>[2x]MAIVKATDQSFSAETSEGVVLADFWAPWCGPSKMIAPVLEELDQEMGDKLKIVKIDVDENQETAGKYGVMSIPTLLVLKDGEVVETSVGFKPKEALQELVNKHLLEHHHHHH

Thioredoxin is a ubiquitous protein that is present in nearly all known organisms from archaea to humans. In its active site, thioredoxin has two cysteine residues in a conserved amino acid motif Trp-Cys-Gly-Pro-Cys, which is a defining characteristic of thioredoxins. Importantly, the lower pKa value of the N-terminal cysteine of thioredoxin promotes its existence as a thiolate, the reactive deprotonated form of thiol, and this thiolate can act as a nucleophile to combine with a protein substrate, resulting in a covalently linked mixed disulfide (thioredoxin–S–S–protein).

Here we present the first structure of a BsTrxA C32S homodimer at 1.5 Å resolution. The C32S BsTrxA homodimer has the expected thioredoxin fold, with a central hydrophobic core with a four-stranded β sheet surrounded by five α helices on the external surface. Importantly, C32S TrxA does indeed crystallize as a dimer held together by a disulfide bond between the two active sites attacking Cys29 residues. In addition, dimerization is facilitated by intermolecular hydrogen bonds and hydrophobic interactions. Intermolecular hydrogen bonds occur between the backbone amide nitrogen of Ile72 and the carbonyl of Trp28, and between the backbone carbonyl of Ile72 and the amide nitrogen of Gly30. The large hydrophobic residue Trp28, which precedes the catalytic Cys29, interacts with a shallow hydrophobic pocket on the other chain consisting of the side chains of Ala26, Trp28, Val57, Ala64, Val69, and Ile72. The crystal structure shows that the side chain of the mutated residue C32S points away from the intermolecular disulfide Cys29-Cys29 bond, forming hydrogen bonds to the backbone amide of Ala26 and the carbonyls of Ala26 or Cys29. The C32S BsTrxA homodimer structure described here, however, has the same peptide chain orientation as the NF-κB peptide. In the BsTrxA homodimer structure described here, only two of these loops are involved in the interactions; the third loop (residues 88–91) does not interact with the other chain of the dimer. Taken together, our present structural analysis of the C32S BsTrxA dimer indicates that the high-resolution structure obtained in this study can serve to visualize a mixed disulfide intermediate state in the thiol–disulfide exchange reaction catalyzed by the native enzyme.> GAGCAGACGTGACACCACTCA;> TGTCA;> TCTGAGTGG;> CGTCTGC

In this work, we exhaustively probe the ability of all 36 immobile HJ sequences to form DNA crystals in two different designed systems. Three separate self-assembling DNA crystal systems are described in this report: the “4 × 5” and “4 × 6” designs (collectively referred to as the 4 × N systems), and a third construct with a “scrambled” sequence variant of the 4 × 6 lattices. Self-assembly was mediated by three constituent oligonucleotides: (S1) containing four sequence repeats of either 5 or 6 bases; (S2) composed of 21 bases containing complementary regions to both (S1); and (S3) which forms the second junction crossover. The HJ serves as the fundamental component at the core of each unit, and the ultimate assembly of the full lattice is facilitated by the complementary 2-base sticky ends that tail each duplex.

The 4 × 5 system robustly crystallized with 75% of the junctions, and we obtained crystals in all but 9 of 36 sequences. Of the resulting structures, 18 exhibited P32 symmetry with average cell dimensions a = b = 68.85 Å c = 60.09 Å, with only nine retaining the original P3221 symmetry with average cell edges a = b = 68.17 Å c = 60.60 Å. Although the cell parameters between the two symmetries were virtually indistinguishable, the differences between the periodicity of the lattices is dramatic, with vastly different cavity sizes. While the highest resolution achieved for the J1 system was 3.1 Å, in roughly half of the crystals measured the resolutions were 3.05 Å or better, and as high as 2.9 Å (J6) and 2.75 Å (J19), for the P32 and P3221 symmetries, respectively. Pos1 and 2 were readily observable in the electron density maps at either one or both of these conserved sites in a significant number of the structures, with no apparent respect to motif or symmetry. However, in the majority of the crystal structures reported here, the cacodylate anion indeed fits best into the electron density map of our X-ray structures, due to the presence of sodium cacodylate in the crystallization solution.>[5x]QANLMRLKSDLFNRSPMYPGPTKDDPLTVTLGFTLQDIVKVDSSTNEVDLVYYEQQRWKLNSLMWDPNEYGNITDFRTSAADIWTPDITAYSSTRPVQVLSPQIAVVT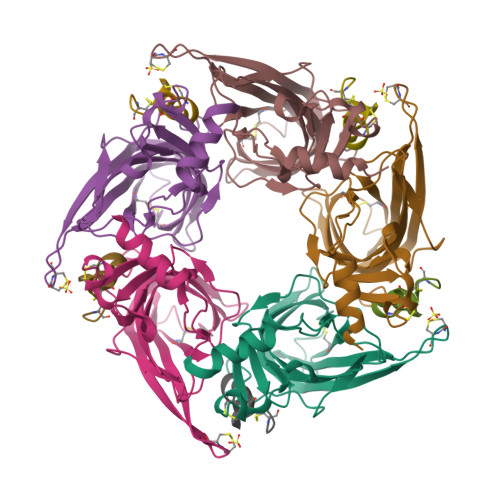HDGSVMFIPAQRLSFMCDPTGVDSEEGVTCAVKFGSWVYSGFEIDLKTDTDQVDLSSYYASSKYEILSATQTRQVQHYSCCPEPYIDVNLVVKFRERRAGNGFFRNLFD;>[5x]GCCSLPPCALNNPKYCX> AHFEKRFLKRIRDLGEGHFGKVELCRYDPEGDNTGEQVAVKSLKPESGGNHIADLKKEIEILRNLYHENIVKYKGICTEDGGNGIKLIMEFLPSGSLKEYLPKNKNKINLKQQLKYAVQICKGMDYLGSRQYVHRDLAARNVLVESEHQVKIGDFGLTKAIETDKEYYTVKDDRDSPVFWYAPECLMQSKFYIASDVWSFGVTLHELLTYCDSDSSPMALFLKMIGPTHGQMTVTRLVNTLKEGKRLPCPPNCPDEV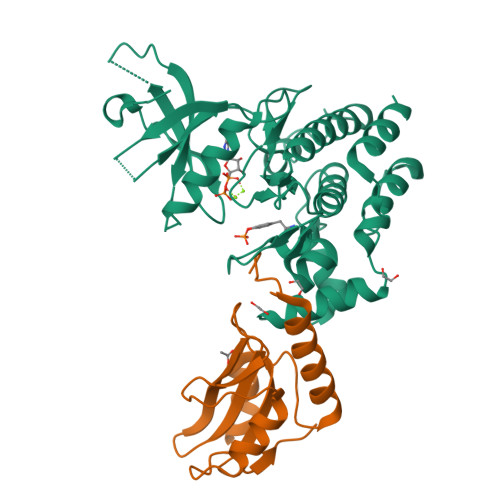YQLMRKCWEFQPSNRTSFQNLIEGFEALL;> STHFRTFRSQADFSSITRASSLLDACGFYWGPLTVSAAHEKLKSEPEGTFLIRDSTQKNCFFAISVKTATGPTSIRINFQTGRFSLDGSKETFDCLFKLLEHYLSSPRKVLVTPLRK>[5x]MSLITVNTLQKMKAAGEKIAMLTAYESSFAALMDDAGVEMLLVGDSLGMAVQGRKSTLPVSLRDMCYHTECVARGAKNAMIVSDLPFGAYQQSKEQAFAAAAELMAAGAHMVKLEGGVWMAETTEFLQMRGIPVCAHIGLTPQSVFAFGGYKVQGRGGKAQALLNDAKAHDDAGAAVVLMECVLAELAKKVTETVSCPTIGIGAGADCDGQVLVMHDMLGIFPGKTAKFVKNF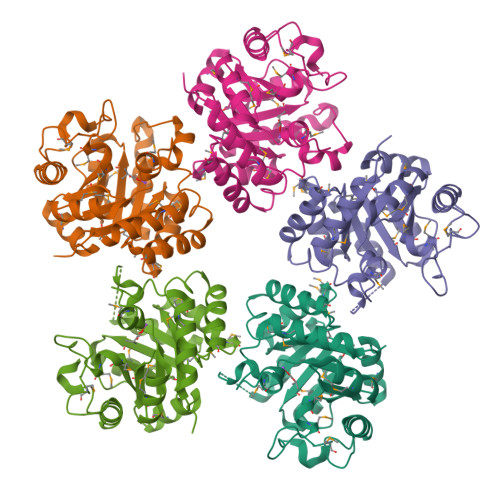MQGHDSVQAAVRAYVAEVKAKTFPAAEHIFADEGGSHHHHHH>[4x]MNLPTAQEVQGLMARXIELVDVGDIEAIVQMYADDATVENPFGQPPIHGREQIAAFYRQGLGGGKVRACLTGPVRASHNGCGAMPFRVEMVWNGQPCALDVIDVM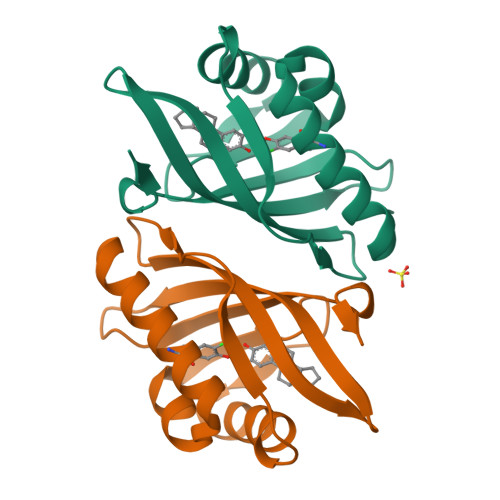RFDEHGRIQTMQAYWSEVNLSVREPQLVPR>MAITSTGLTAKTGVEHFGTVGVAMVTPFTESGDIDIAAGREVAAYLVDKGLDSLVLAGTTGESPTTTAAEKLEL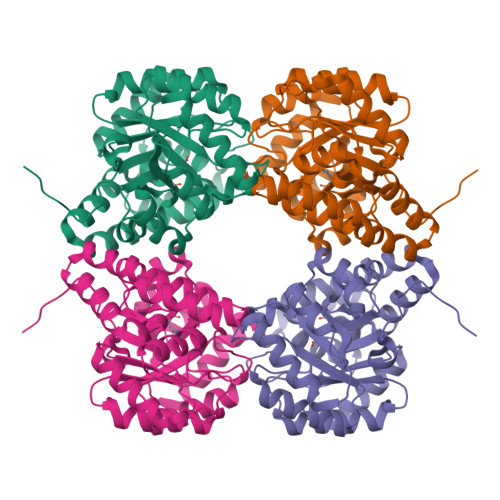LKAVREEVGDRAKLIAGVGTNNTRTSVELAEAAASAGADGLLVVTPYYSKPSQEGLLAHFGAIAAATEVPICLYDIPGRSGIPIESDTMRRLSELPTILAVKDAKGDLVAATSLIKETGLAWYSGDDPLNLVWLALGGSGFISVIGHAAPTALRELYTSFEEGDLVRAREINAKLSPLVAAQGRLGGVSLAKAALRLQGINVGDPRLPIMAPNEQELEALREDMKKAGVL[2x]> MQAHEESQLM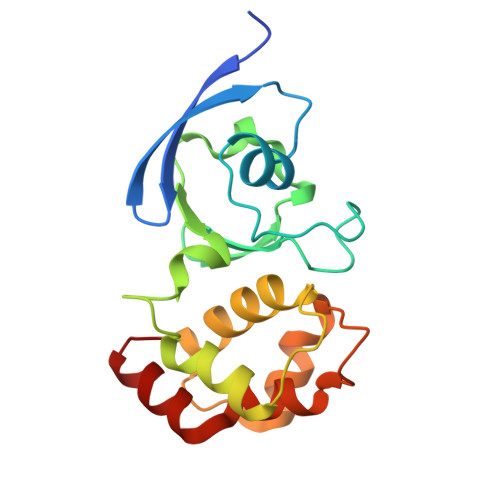RISATINGKPRVFYVEPRMHLADALREVVGLTGTKIGCEQGVCGSCTILIDGAPMRSCLTLAVQAEGCSIETVEGLSQGEKLNALQDSFRRHHALQCGFCTAGMLATARSILAENPAPSRDEVREVMSGNLCRCTGYETIIDAITDPAVAEAARRGEV> SS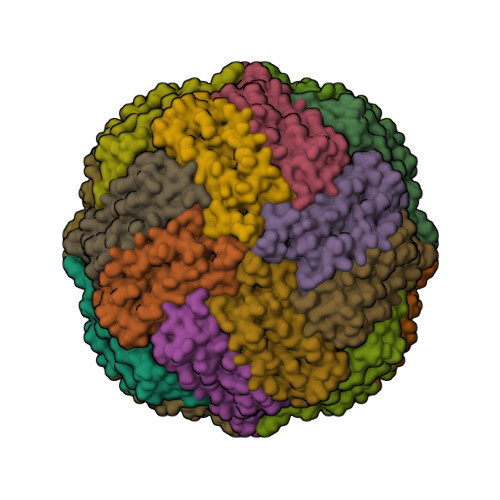QIRQNYSTEVEAAVNRLVNLYLRASYTYLSLGFYFDRDDVALEGVAHFFRELAEEKREGAERLLKMQNQRGGRALFQDLQKPSQDEWGTTLDAMKAAIVLEKSLNQALLDLHALGSAQADPHLCDFLESHFLDEEVKLIKKMGDHLTNIQRLVGSQAGLGEYLFERLTLKHD>[4x]MSKDRMVELLQEHFELNLYEARAYVALVAFGVLTPAELASVSEVPAPRTYDVLRSLEKKGFAMTQPGKTNKYRPVHPANVLEKFIQDWQERVKEELEAKKKAKEELLELMAPLIETEVP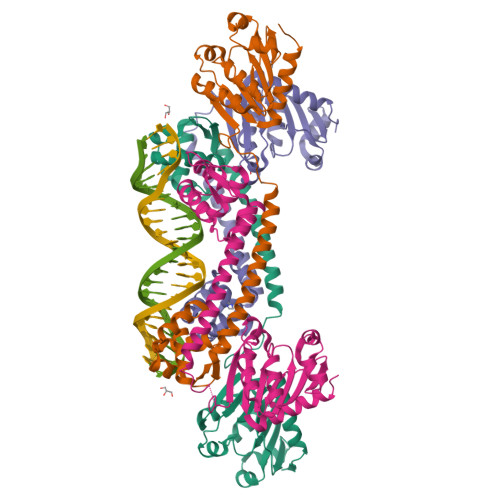KYGVERVWVVRGIKNSTLKTKEMLEEAQNEILLADDGFIAVNLEDDIIKAVDRGVKTKILLTKNLLPRLKASKIIDYAKEGKLELRALDKFDLPMLICDEEVFFALEDLAARYFNYETQVWIKDHRVVALFKEKFNEYWEKAEKV> KDNIRHGVCWI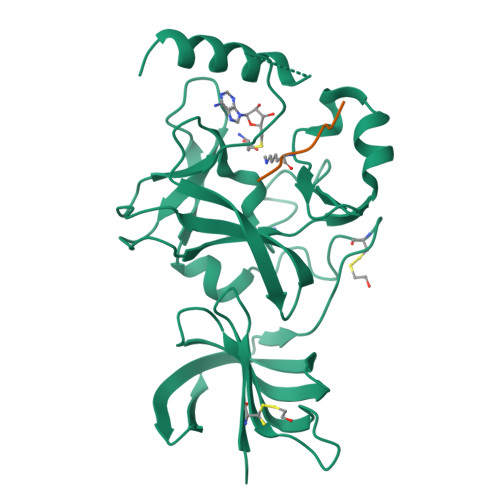YYPDGGSLVGEVNEDGEMTGEKIAYVYPDERTALYGKFIDGEMIEGKLATLMSTEEGRPHFELMPGNSVYHFDKSTSSCISTNALLPDPYESERVYVAESLISSAGEGLFSKVAVGPNTVMSFYNGVRITHQEVDSRDWALNGNTLSLDEETVIDVPEPYNHVSKYCASLGHKANHSFTPNCIYDMFVHPRFGPIKCIRTLRAVEADEELTVAYGYDHSPPGKSGPEAPEWYQVELKAFQATQQK;> IKRSKKNSLA>[3x]SSSESHIFIYGGCSPEKYTPNTPFESNRDTFLSSVVTSSSDASFNSFAV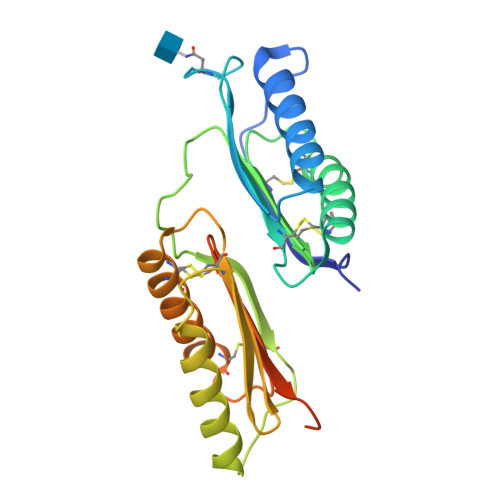GNDSSSSSSSSAVFGLYQCRDDLRSSDCSKCIQTSVDQITLICPYSYGASLQLEGCFLRYETNDFLGKPDTSLRYKKCSSKSVENDYDFFKRRDDVLSDLESTQLGYKVSRSGLVEGYAQCVGDLSPSDCTACLAESVGKLKNLCGSAVAAEVYLAQCYARYWGSGYYDFSSDPTNGDHVGKSLEGSENLYFQ For this bacterium, Feo is the primary system that transports Fe2+ into the cytosol. FeoA and FeoC are known to be small (ca. 7–10 kDa) cytosolic proteins, while FeoB is a large (ca. 80–100 kDa) polytopic transmembrane protein that contains an N-terminal soluble G-protein-like domain termed NFeoB. The status of GTP and GDP bound to the NFeoB region is hypothesized to control the opening and closing of the FeoB pore and therefore the translocation of Fe2+ into the bacterial cytosol.

Partial sequence alignments revealed that the position analogous to Asn150 within the G5 motif of the VcNFeoB NTPase domain is highly variable for NFeoBs known to be NTPases, while this same position is an invariant Thr residue for NFeoBs known to be strict GTPases. To test the structural basis of this hypothesis, we expressed, purified, and crystallized the G5 motif N150T variant of VcNFeoB(His)6 in the presence of GDP. The crystals diffracted to 2.9 Å resolution, and initial analysis revealed one apo VcNFeoB(His)6 NTPase domain and one GDP-bound VcNFeoB(His)6 NTPase domain both within the asymmetric unit. This hetero-oligomerization is likely crystallization induced based on our in-solution studies. Omit maps confirmed that substantial density was present and consistent with GDP in one, but not both, molecules within the asymmetric unit, allowing us to visualize a direct comparison between the apo and the GDP-bound N150T variant at the same resolution. Interestingly, the presence of Thr in position 150 affects the hydrogen bonding pattern surrounding the guanine nucleobase both directly and indirectly. First, the Thr hydroxyl moiety now makes a new hydrogen bond with position N1 along the purine ring. Second, the removal of Asn150 releases Asp122 to tighten and extend its hydrogen bonds with positions N1 and the H2N-C1 group. However, by comparison to the WT protein, the N150T variant appears to have two key additional hydrogen bonds surrounding the guanine purine that could affect nucleotide stability and may afford the discrimination of GTP relative to other NTPs. Our structure of N150T VcNFeoB(His)6 revealed increased H-bonding to the nucleobase due to the presence of Thr150 in the G5 motif, but this modification alone did not dramatically alter the binding affinity between NFeoB and GDP and only modestly increased the binding affinity between NFeoB and GMP-PNP.

>[2x]MKYQVLTVGNPNSGKTTLFNGLTGAKQQVGNWAGVTVEKKTGSFVHAGDEFSLTDLPGIYALDSGNDSNSIDESIASRAVLTHPADVIINVVDATCLERSLYMTLQLRELRRPMIVVLNKMDALKRERVHLDLKQLEAFLGCPVLALSATNKEQVRRFKEKLHKLLVQGIALKQIELHYGAEFESLIHELEPMFAEQAVSARALAIRALENDRLVINGLKEAERQNVEQRQHECQVDIDLLVANVRYTYLHELCTHVRRT>[4x]HHHHHHGGTILVVTGTGTGVGKTVVCAALASAARQAGIDVAVCKPVQTGTARGDDDLAEVGRLAGVTQLAGL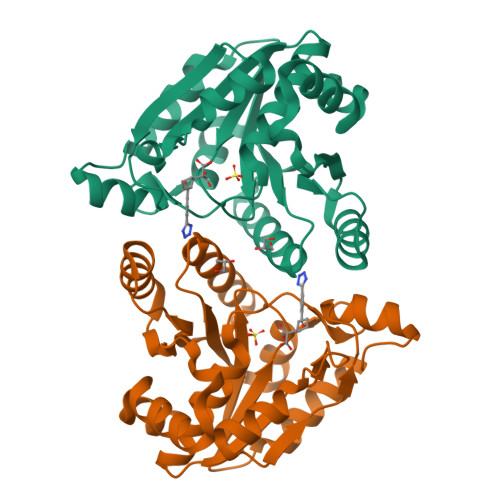ARYPQPMAPAAAAEHAGMALPARDQIVRLIADLDRPGRLTLVEGAGGLLVELAEPGVTLRDVAVDVAAAALVVVTADLGTLNHTKLTLEALAAQQVSCAGLVIGSWPDPPGLVAASNRSALARIAMVRAALPAGAASLDAGDFAAMSAAAFDRNWVAGLVG> LGKFSQTCYNSAIQGSVLTSTCERTNGGYNTSSIDLNSVIENVDGSLKWQGSNFIETCRNTQLAGSSELAAECKTRAQQFVSTKINLDDHIANIDGTLKY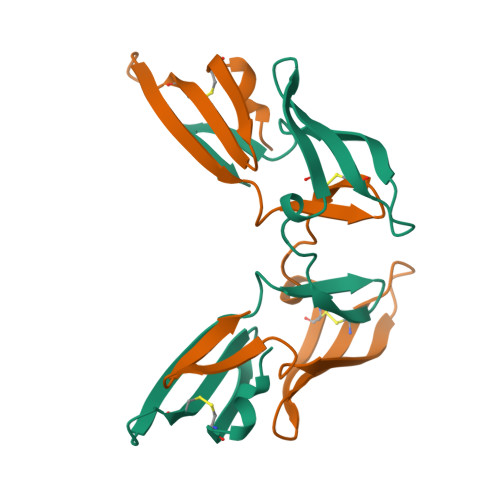E> MDSATTESLRAATHDVLAGLTAREAKVLRMRFGIDMNTDYTLEEVGKQFDVTRER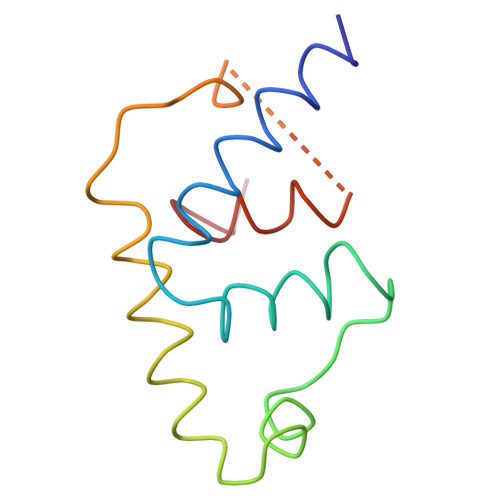IRQIEAKALRKLRHPSRSEVLRSGSSGSGTPEEKLLRAIFGEKA>[2x]MPNFSG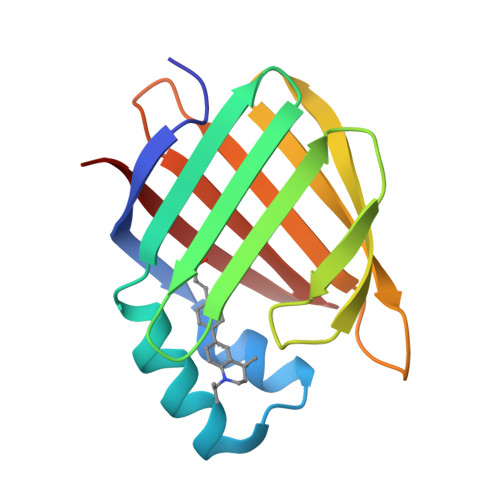NWKIIRSENFEELLKVLGVNVMLRKIAVAAASKPAVEIKQEGDTFYIKTSTTVRTTEINFKVGEEFEEQTVDGRPCKSLVKWESENKMVCEQKLLKGEGPKTSWTRELTNDGELILTMTADDVVCTRVYVRE>[2x]MKKLKVMTVFGTRPEAIKMA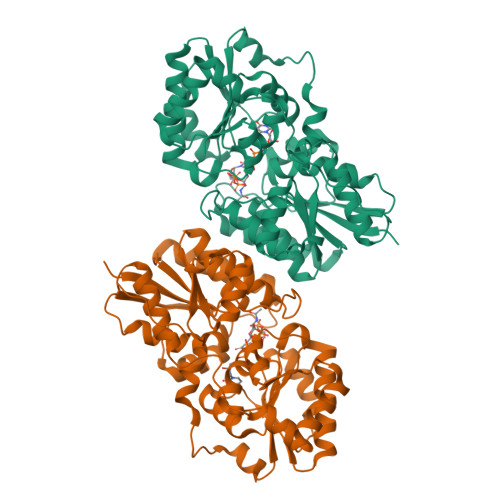PLVLELKKYPEIDSYVTVTAQHRQMLDQVLDAFHIKPDFDLNIMKERQTLAEITSNALVRLDELFKDIKPDIVLVHGDTTTTFAGSLAAFYHQIAVGHVEAGLRTGNKYSPFPEELNRQMTGAIADLHFAPTGQAKDNLLKENKKADSIFVTGNTAIDALNTTVRDGYSHPVLDQVGEDKMILLTAHRRENLGEPMENMFKAIRRIVGEFEDVQVVYPVHLNPVVREAAHKHFGDSDRVHLIEPLEVIDFHNFAAKSHFILTDSGGVQEEAPSLGKPVLVLRDTTERPEGVEAGTLKLAGTDEENIYQLAKQLLTDPDEYKKMSQASNPYGDGEASRRIVEELLFHYGYRKEQPDSFTGKLEHHHHHH>[2x]MRGSAHVVILGAGTGGMPAAYEMKEALGSGHEVTLISANDYFQFVPSNPWVGVGWKERDDIAFPIRHYVERKGIHFIAQSAEQIDAEAQNITLADGNTVHYDYLMIATGPKLAFENVPGSDPHEGPVQSICTVDHAERAFAEYQALLREPGPIVIGAMAGASCFGPAYEYAMIVASDLKKRGMRDKIPSFTFITSEPYIGHLGIQGVGDSKGILTKGLK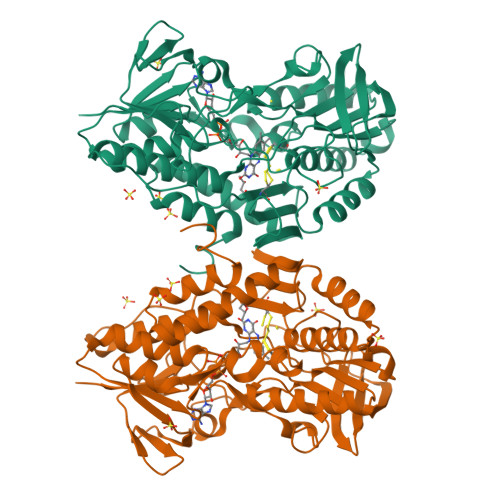EEGIEAYTNCKVTKVEDNKMYVTQVDEKGETIKEMVLPVKFGMMIPAFKGVPAVAGVEGLCNPGGFVLVDEHQRSKKYANIFAAGIAIAIPPVETTPVPTGAPKTGYMIESMVSAAVHNIKADLEGRKGEQTMGTWNAVCFADMGDRGAAFIALPQLKPRKVDVFAYGRWVHLAKVAFEKYFIRKMKMGVSEPFYEKVLFKMMGITRLKEEDTHRKAS> NTTDTLF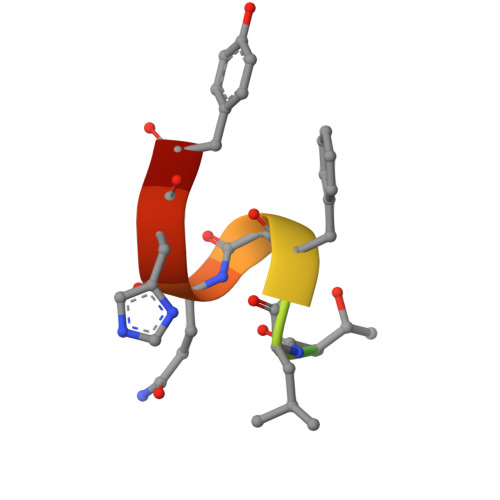SQHYR>LERGRDYEKNKVCKEFSHLGKEDFTSLSLVLYSRKFPSGTFEQVSQLVKEVVSLTEACCAEGADPDCYDTRTSALSAKSCESNSPFPVHPGTAECCTKEGLERKLCMAALKHQPQEFPTYVEPTNDEICEAFRKDPKEYANQFMWEYSTNYGQAPLSLLVSYTKSYLSMVGSCCTSASPTVCFLKERLQLKHLSLLTTLSNRVCSQYAAYGEKKSRLSNLIKLAQKVPTADLEDVLPLAEDITNILSKCCESASEDCMAKELPEHTVKLCDNLSTKNSKFEDCCQEKTAMDVFVCTYFMPAAQLPELPDVELPTNKDVCDPGNTKVMDKYTFELSRRTHLPEVFLSKVLEPTLKSLGECCDVEDSTTCFNAKGPLLKKELSSFIDKGQELCAD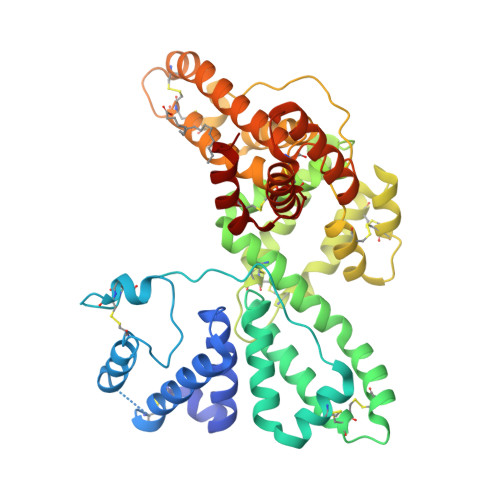YSENTFTEYKKKLAERLKAKLPDATPTELAKLVNKRSDFASNCCSINSPPLYCDSEIDAELKNIL[2x]> RICFNHQGSQPQTTKTCSPGESSCYNKQWSDFRGTIIERGCGCPTVKP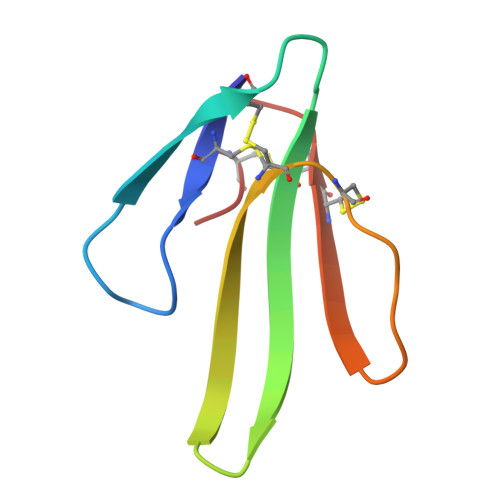GIKLSCCESEVCNN>ETGDSIIHIGAIFEENAAKDDRVFQLAVSDLSLNDDILQSEKITYSIKVIEANNPFQAVQEACDLMTQGILALVTSTGCASANALQSLTDAMHIPHLFVQRNPGGSPRTACHLNPSP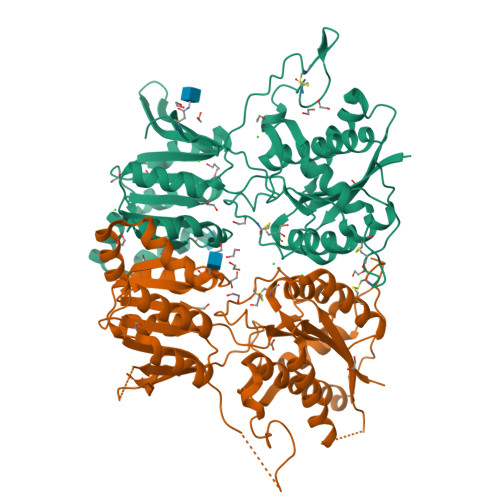DGEAYTLASRPPVRLNDVMLRLVTELRWQKFVMFYDSEYDIRGLQSFLDQASRLGLDVSLQKVDKNISHVFTSLFTTMKTEELNRYRDTLRRAILLLSPQGAHSFINEAVETNLASKDSHWVFVNEEISDPEILDLVHSALGRMTVVRQIFPSAKDNQKCMRNNHRISSLLCDPQEGYLQMLQISNLYLYDSVLMLANAFHRKLEDRKWHSMASLNCIRKSTKPWNGGRSMLDTIKKGHITGLTGVMEFREDSSNPYVQFEILGTTYSETFGKDMRKLATWDSEKGLNGSLQERPMGSRLQGGTKHHHHHH[3x]>[12x]MAMAQELTAMSAWVNQDGSTLYINSINAQGELTGSYINRAAGFACQNSPYPVNGWVFGTAISFS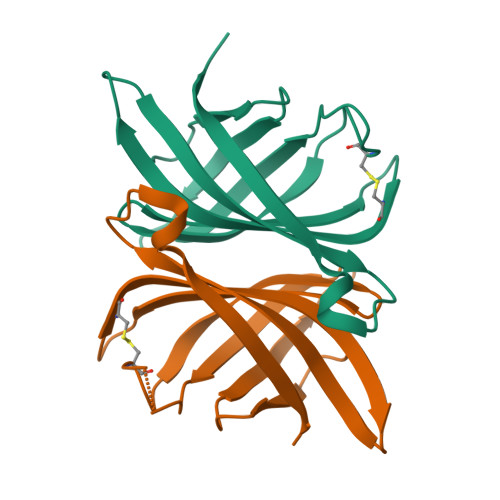TKWLNSVESCNSITSWSGFYINTGGQGKISTLWQLVVNGSSSPSQILKGQDVFSQTSA>[2x]GAPQEMYAPHSIRIEGDVTLGGLFPVHAKGPSGVPCGDIKRENGIHRLEAMLYALDQINSDPNLLPNVTLGARILDTCSRDTYALEQSLTFVQALIQKDTSDVRCTNGEPPVFVKPEKVVGVIGASGSSVSIMVANILRLFQIPQISYASTAPELSDDRRYDFFSRVVPPDSFQAQAMVDIVKALGWNYVSTLAS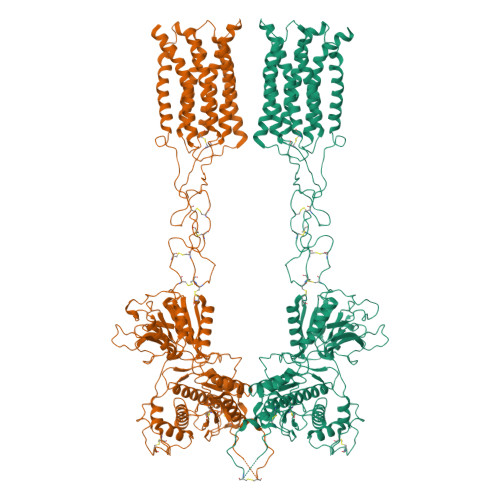EGSYGEKGVESFTQISKEAGGLCIAQSVRIPQERKDRTIDFDRIIKQLLDTPNSRAVVIFANDEDIKQILAAAKRADQVGHFLWVGSDSWGSKINPLHQHEDIAEGAITIQPKRATVEGFDAYFTSRTLENNRRNVWFAEYWEENFNCKLTISGSKKEDTDRKCTGQERIGKDSNYEQEGKVQFVIDAVYAMAHALHHMNKDLCADYRGVCPEMEQAGGKKLLKYIRNVNFNGSAGTPVMFNKNGDAPGRYDIFQYQTTNTSNPGYRLIGQWTDELQLNIEDMQWGKGVREIPASVCTLPCKPGQRKKTQKGTPCCWTCEPCDGYQYQFDEMTCQHCPYDQRPNENRTGCQDIPIIKLEWHSPWAVIPVFLAMLGIIATIFVMATFIRYNDTPIVRASGRELSYVLLTGIFLCYIITFLMIAKPDVAVCSFRRVFLGLGMCISYAALLTKTYRIYRIFEQGKKSVTAPRLISPTSQLAITSSLISVQLLGVFIWFIVDPPNIIIDYDEHKTMNPEQARGVLKCDITDLQIICSLGYSILLMVTCTVYAFKTRGVPENFNEAKYIGFTMYTTCIVWLAFIPIFFGTAQSAEKLYIQTTTLTISMNLSASVALGMLYMPKVYIIIFHPELNVQKREFLEVLFQGPGSGSWSHPQFEKDYKDDDD>[4x]WEETKECAFTEFFKLAPLASNPALSVCQDASGWQMLPPAGYPTPEQLKLMCGTAECFT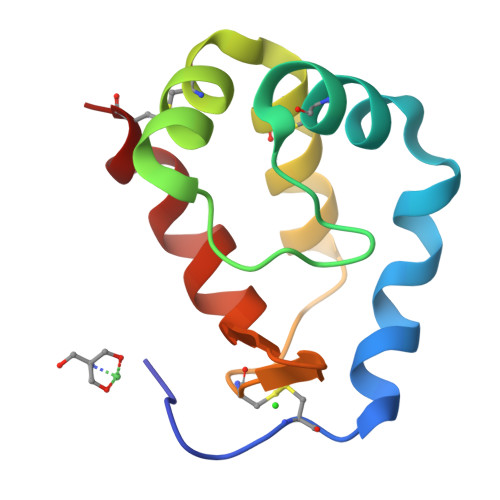LIDAIKALNPNDCILVFGDVRLNVKKLVTEFEPSCF> MTPPKAEKRPYPITTHGDTRVDDYYWLRDDERTDPQVLDYLQAENAFTDAALKPQQALRETLYEEMVARENLYFQSVPYVRHGYRYQTRFEPGNEYAIYVRQPQAESEHWDTLIDGNQRAEQRAFYTLGGLEVSPDNQKLAVAEDFLSRRQYDIRFKNLSDDSWTDEVLENTSGSFEWANDSATVYYVRKHAKTLLPYQVYRHVVGTDPQLDELIYEEQDDTFYVGLEKTTSDRFILIHLSSTTTSEILLLDADRADSTPQMFVPRRKDHEYGIDHYHQHFYIRSNKDGKNFGLYQSEQADEAQWQTLIAPRIEVMLEGFSLFRDWLVVEERSEGLTQLRQIHWQ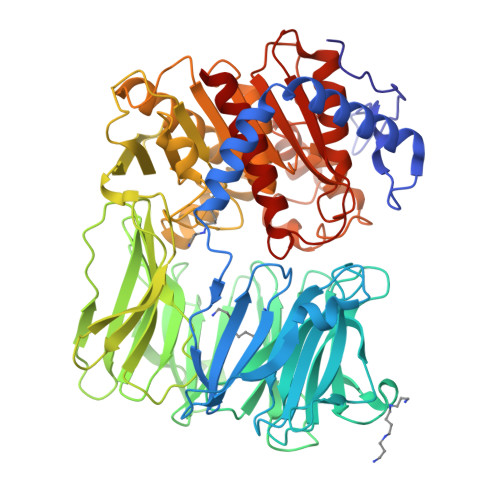SGEVKRIAFDDPTYTTWLAYNPEPETELLRYGYSSMTTPTTLYELNLDSDERVMLKQQEVKNFTPENYRSERVWVKARDGVEVPVSLVYRHDSFARGTNPLMVYGYGSYGSSMDPAFSASRLSLLDRGFVFVLAHIRGGGELGQLWYEDGKLFKKQNTFNDFIDVTEALIAQGYGDAKRVFAMGGSAGGLLMGAVINQAPELFNGIVAQVPFVDVVTTMLDESIPLTTGEYDEWGNPNQQAYYDYILQYSPYDQVKAQDYPHMLVTTGLHDSQVQYWEPAKWVAKLRELKTDDRQLLLYTDMDSGHGGKSGRFKAYEDIALEYAFILALAE>[3x]MTTADLILINNWYVVAKVEDCRPGSITTAHLLGVKLVLWRSHEQNSPIQVWQDYCPHRGVPLSMGEVANNTLVCPY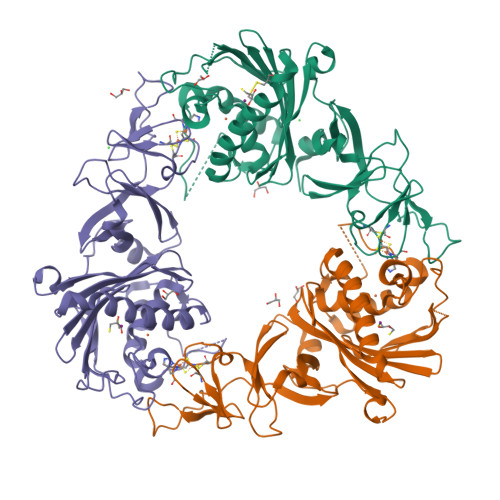HGWRYNQAGKCVQIPAHPDMVPPASAQAKTYHCQERYGLVWVCLGNPVNDIPSFPEWDDPNYHKTYTKSYLIQASPFRVMDNSIDVSHFPFIHEGILGDRNHAEVEDLEVKVDKDGLTMGKYQVHTSKFNNSTKDDSMVNWFRLSHPLCQYCSTEASEMRTVDLMVVTPIDEDNSVLRYLIMWNGSKTLESKILADYDQVIEEDIRILHSQQPTRLPLLSPKQINTQGLPQEIHVPSDRCTVAYRRWLKELGVTYGVC ethyl methyl 4-(2,3-dichlorophenyl)-2,6-dimethylpyridine-3,5-dicarboxylate | C18 H17 Cl2 N O4 | 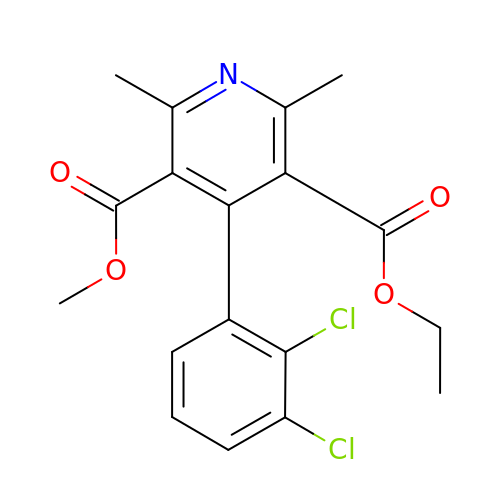REQRUBNOOIAHMG-UHFFFAOYSA-N> AAPDEITTAWPVNVGPLNPHLATPNQMFAQSMVYEPLVKYQADGSVIPWLAKSWTHSEDGKTWTFTLRDDVKFSNGEPFDAEAAAENFRAVLDNRQAHAALELANQIVDVKALSKTELQITLKSAYYPFLQELALPAPFRFIAPSQFKNHETMNGIKAPIGTGPWILQESKLNQYDVFVRNENYWGEKPAIKKITFNVIPDPTTRAVAFETGDIDLLYGNEGLLPLDTFARFSQNPAYHTQLSQPIETVMLALNTAKAPTNELAVREALNYAVNKKSLIDNALYGTQQVADTLFAPSVPYANLGLKPSQYDPQKAKALLEKAGWTLPAGKDIREKNGQPLRIELS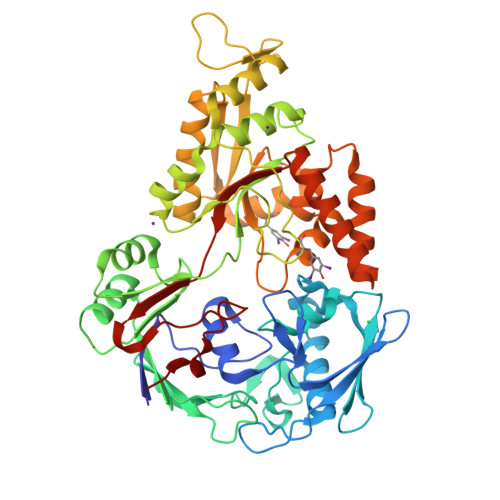FIGTDALSKSMAEIIQADMRQIGADVSLIGEEESSIYARQRDGRFGMIFHRTAGAPADPHAFLSSMRVPSHADFQAQQGLADKPLIDKEIGEVLATHDETQRQALYRDILTRLHDEAVYLPISYISMMVVSKPELGNIPYAPIATEIPFEQIKPVKP4-cyclopropyl-7-fluoro-3,4-dihydro-2H-1,2,4-benzothiadiazine 1,1-dioxide | C10 H11 F N2 O2 S | 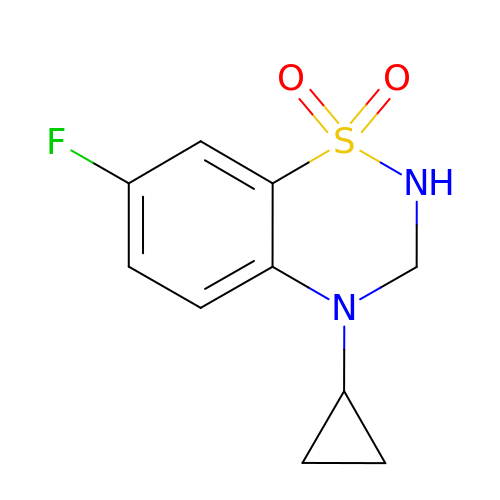FLTMTBPCYAZIKM-UHFFFAOYSA-N> MRTFFVGGNWKANPKTVEEAEKLIEMLNGAKVEGNVEVVVAAPFGFLPTLQQKLRKDWKVSAENVFTKPNGAFTGEVTVPMIKSFGIEWTILGHSERRDILKEDDEFLAAKAKFALENGMKIIYCCGEHLSEREAGKASEFVSAQIEKMIPAIPAGKWDDVVIAYEPIWAIGTGKVASTQDAQEMCKVIRDILAAKVGADIANKVRILYGGSVKPNNCNELAACPDVDGF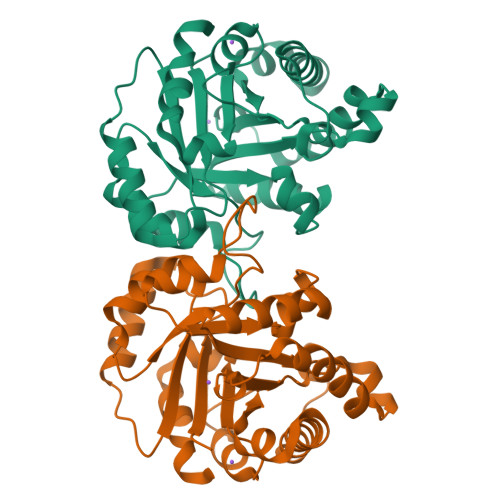LVGGASLEPGFINIVNSNVHSK>MNNSFLDKLIETKELKNSLYNVLKHNFLYHANKIAGSTFTTEALALLLDKNVVTGRHTLDDVQETVNSSYVFDTVIDSLKEKITHNFLRNLHSSLIFNTTLHSRGMAGIYKTIPNMILGTDVSIAQPFEVEPKLDELIEWYYSQSEVSIKVIAEFHYRFELIHPFQDGNGRIGRFVMLKQMLENNLPIKIVSWDSE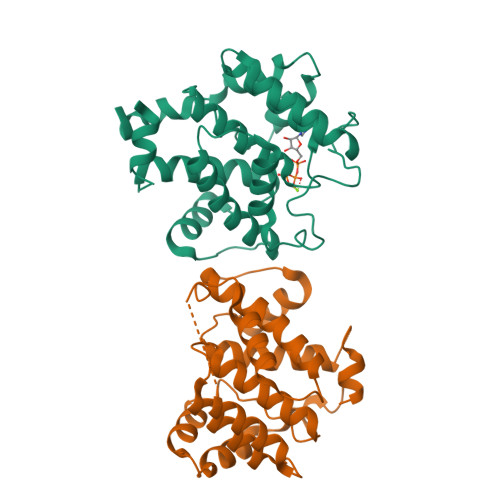DLYRNSLNSCSLGNYVPLIEYLSSLEDFREVYKMLWKLE[4x]>MNHKVHHHHHHIEGRHMVSVEEIRK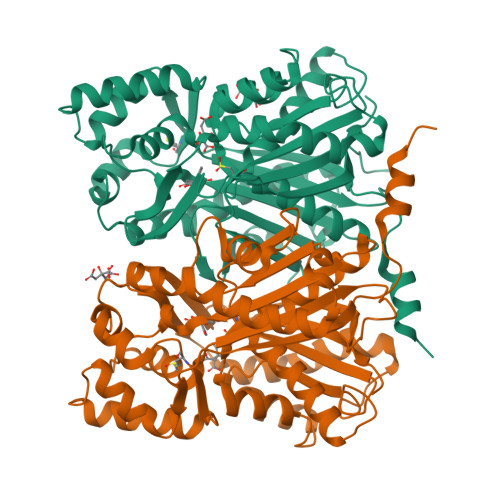AQRAEGPATVMAIGTATPPNCVDQSTYPDYYFRITNSEHMTELKEKFKRMCDKSMIKKRYMYLNEEILKENPSVCAYMAPSLDARQDMVVVEVPKLGKEAATKAIKEWGQPKSKITHLIFCTTSGVDMPGADYQLTKLLGLRPSVKRYMMYQQGCFAGGTVLRLAKDLAENNKGARVLVVCSEITAVTFRGPTDTHLDSLVGQALFGDGAAAVIVGSDPLPVEKPLFQLVWTAQTILPDSEGAIDGHLREVGLTFHLLKDVPGLISKNIEKALVEAFQPLGISDYNSIFWIAHPGGPAILDQVEAKLGLKPEKMEATRHVLSEYGNMSSACVLFILDQMRKKSIENGLGTTGEGLDWGVLFGFGPGLTVETVVLRSVTL[2x]>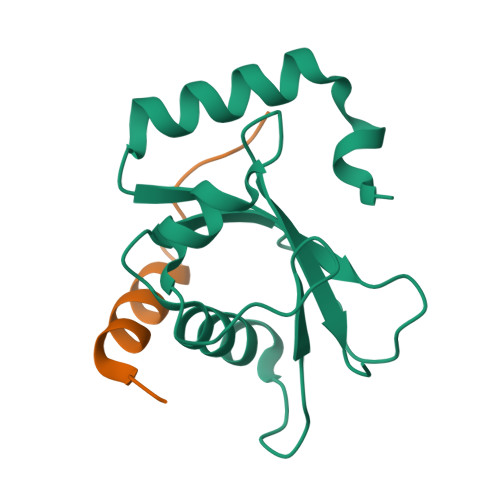 GPHMRSQFKDDFSFEKRKTESQRIREKYPDRIPVICEKVDKSDIAAIDKKKYLVPSDLTVGQFVYVIRKRIKLSPEKAIFIFIDEILPPTAALMSTIYEEHKSEDGFLYITYSGENTFG;> MLQFEIDDEMEPLYNQAKQMRYGDYLEVLFQ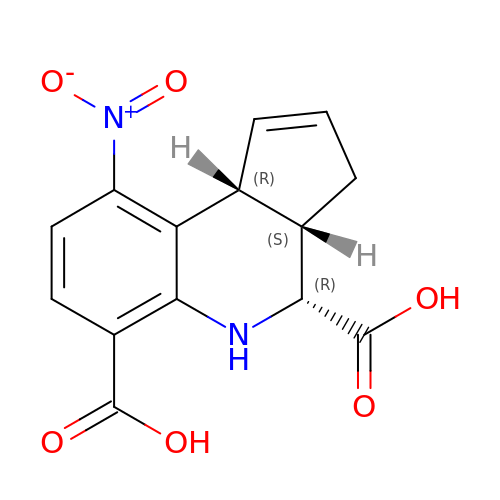(3aS,4R,9bR)-9-nitro-3a,4,5,9b-tetrahydro-3H-cyclopenta[c]quinoline-4,6-dicarboxylic acid | C14 H12 N2 O6 | CTXNQOWRJIPUOM-KEHGIVTQSA-N>[2x]GAMNPDPEATMDRSLLQRQDLPYRFSAVDLDSVDGQRHYRLWLGRPLQAPPAAGYPVVWMLDGNAAVGALDESTLRRLADGDAPLLVAIGYRTPLRIDRAGRTFDYTPASPGQADQRDPLNGLPSGGADAFLDLLRDGMRPAVAAQAPLDTARQTLWGHAYGGLLVLHALFTRPGEFARYAAASPSLWWRDGAILGERAGLEQRLRGKRAELLLWRGSAEPASPRGSLKAEPGQA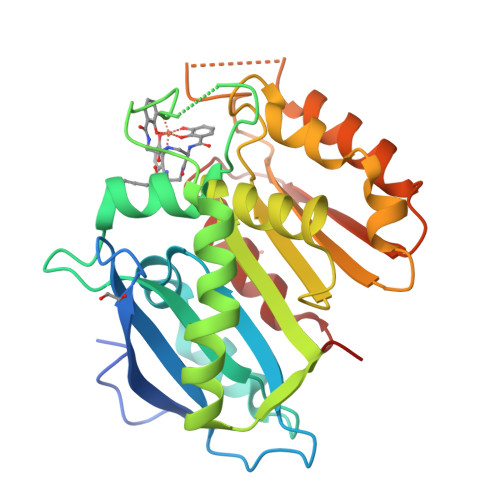MARLVDDLRRVAGLTLDFQPLDGLGHGETLGASLRLLLARPAVERQR N-{4-[(6aR)-3-amino-1,9-dioxo-1,2,5,6,6a,7-hexahydroimidazo[1,5-f]pteridin-8(9H)-yl]benzene-1-carbonyl}-L-glutamic acid | C20 H21 N7 O7 | 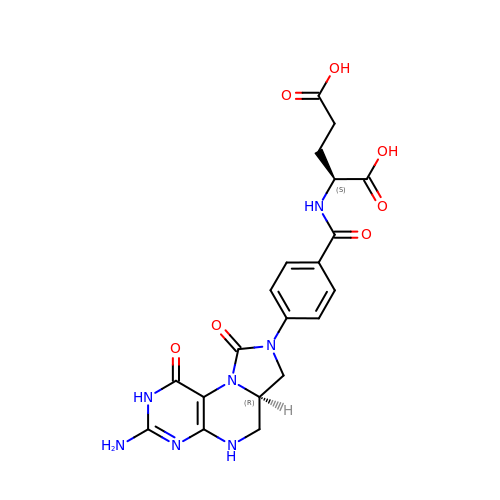JSNFRYBHBVDHSG-NEPJUHHUSA-N> ATFLIWPIYPKIEANEKATAVWLQNTGKTDAMVQIRVFKWNQDGLKDNYSEQSEIIPSPPVAKIKAGEKHMLRLTKSVNLPDGKEQSYRLIVDELPIRLSDGNEQDASKVSFQMRYSIPLFAYGKGIGSGLTEESQKLNAKNALAKPVLQWSVRNNQQGQSELYLKNNGQKFARLSALKTSKTGNDISLGKAAFGYVLSNSTVKFAIDQSTAHELAKTSKIYGVDSSGIKQELIE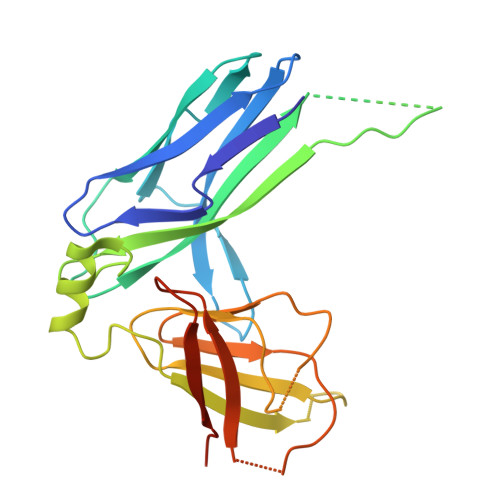ITKMEDPSGHHHHHH> GAMEEDERGKLFVGGLSWETTQENLSRYFCRFGDIIDCVVMKNN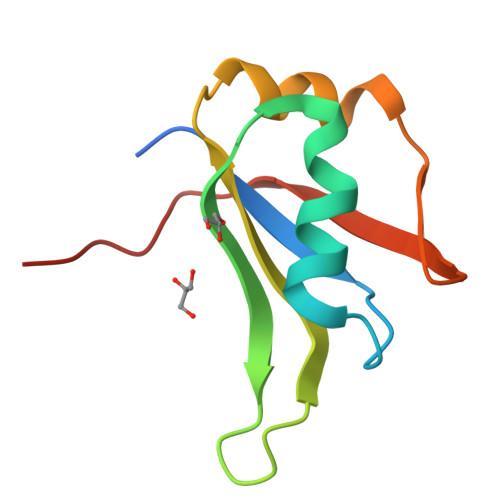ESGRSRGFGFVTFADPTNVNHVLQNGPHTLDGRTIDPKPCNPRTLQ> MRVLVTGGSGYIGSHTCVQLLQNGHDVIILDNLCNSKRSVLPVIERLGGKHPTFVEGDIRNEALMTEILHDHAIDTVIHFAGLKAVGESVQKPLEYYDNNVNGTLRLISAMRAANVKNFIFSSTATVYGDNPKIPYVESFPTGTPQSPYGKSKLMVEQILTDLQKAQP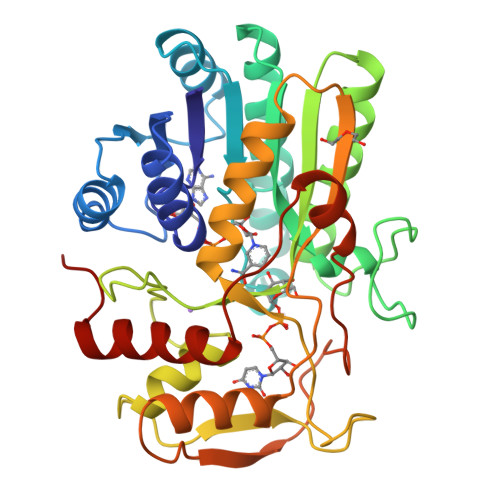DWSIALLRYFNPVGAHPSGDMGEDPQGIPNNLMPYIAQVAVGRRDSLAIFGNDYPTEDGTGVRDYIHVMDLADGHVVAMEKLANKPGVHIYNLGAGVGNSVLDVVNAFSKACGKPVNYHFAPRREGDLPAYWADASKADRELNWRVTRTLDEMAQDTWHWQSRHPQGYPD6-[4-(5-chloranyl-1~{H}-indol-3-yl)piperidin-1-yl]carbonyl-4~{H}-1,4-benzoxazin-3-one | C22 H20 Cl N3 O3 | 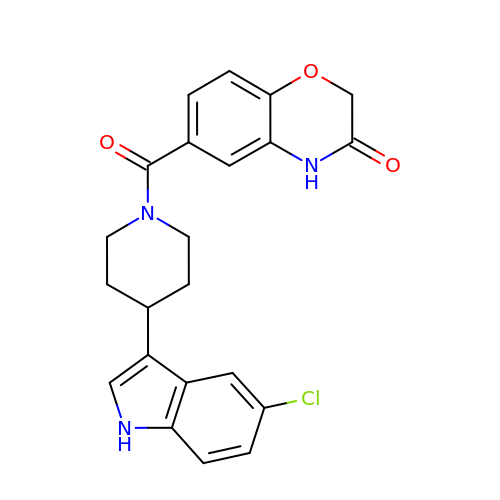NRFBMOTXWSHNOV-UHFFFAOYSA-N>[2x]MRKNFKAFVALFAAILLFFSGCSSKQEAKAPKSEVIYQVMVDRFYNGDPSNDDPEVSKGMFDPTHTNWRMYWGGDLKGLTEKIPYIKGMGVTAIWISPVVDNINKPAVYNGEINAPYHGYWARDFKRVEEHFGTWEDFDNFVKVAHENGIKVILDFAPNHTSPADEENPDFAENGALYDDGKLLGTYSNDSLKLFHHNGSISNWNNLKELQDKNLFDLADLDQSNPIVDKYLKDSIKLWFNHEIDGVRLDAAKHMPMEWVKSFANTIYSIKKDVLLFGEWMLSGPTDPLYGYNIQFANTTGFSVLDFMLNGAIRDVFGKGYGFERLNDTLEDTNKDYENPYKLVTFIDNHDMPRFLSLNNDKDKLHEAIAFIMTTRGIPVIYYGTEQYLHNDTNGGNDPYNRPMMEKFDESTKAYTLIKELSRLRQLTPALQYGTTTARYVSDDVYIYER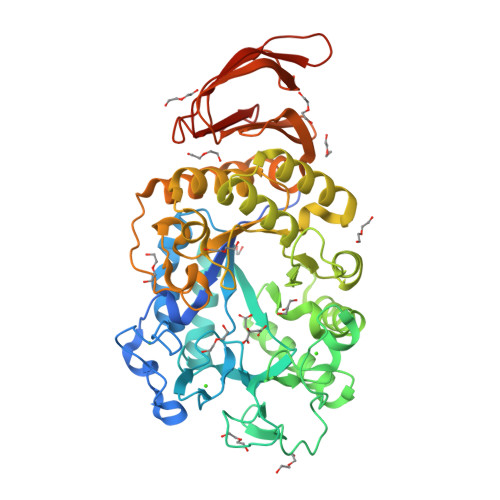QYGKDVVLVAINKGEKTTVKTVKTSLRKGIYKDYLKGLLKGVELKVTKGNGENLVQDLTLPGNSVSVWTNVRVKAAALEHHHHHH(4-bromo-3-cyclopropyl-1H-pyrazol-1-yl)acetic 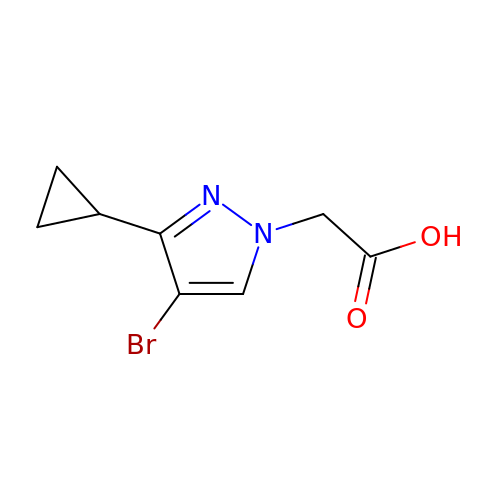acid | C8 H9 Br N2 O2 | DLIOLRMWZAEYPN-UHFFFAOYSA-N>SSTPLSPTRITRLQEKEDLQELNDRLAVYIDRVRSLETENAGLRLRITESEEVVDFYFGKLRNIELICQENEGENDPVLQRIVDILYATDE[4x]

Lamins represent a distinct class within the intermediate filament (IF) protein family. Lamin A (LA) and its splice variant lamin C as well as two closely related lamins B1 and B2 jointly form the lamina, a meshwork of ~3.5-nm-thick filaments located at the inner side of the nuclear envelope. Like for the whole IF family, the basic constitutive unit of the lamin filament is a rod-like dimer which results from a parallel coiled-coil (CC) structure. In line with this, the primary structure of lamins reveals a central α-helical domain responsible for the CC formation which is flanked by non-helical N- and C-terminal domains called the head and the tail respectively.

Crystallographic data for the LA 17-70-Eb1 fusion construct were phased by molecular replacement, relying on the dimeric Eb1 cap as a search model. The crystal structure was refined to 1.83 Å resolution. The asymmetric unit of the crystal contains two copies of the dimer that are readily superimposable. In line with the design, a continuous CC with regular left-handed geometry is formed all along the length of the chimera. Importantly, the structure gives a glimpse of the interface between the head domain and coil1A, as reliable electron density starting with residue 23 is seen in all four chains. The first α-helical residue is Arg28, which is in line with earlier predictions. Interestingly, the side chain of Thr27 stabilizes the N-terminus of the α-helix by making a hydrogen bond with the main-chain nitrogen of Gln30. First, residues 23 through 27 corresponding to the proximal residues of the head domain form a β-strand, facilitated by a Pro residue in position 23. Two such strands form a short antiparallel β-sheet, further referred to as the ‘β-lock’, which flanks the N-terminus of the CC. The second unexpected feature is that, consistently for both dimers in the asymmetric unit, one of the two chains reveals a sharp ~50° change in the α-helical axis direction (‘kink’) at residue Leu35.> MSAPTPLAEASQIPTIPALSPLTAKQSKGNFFSSNPISSFVVDTYKQLHSHRQSLELVNPGTVENLNK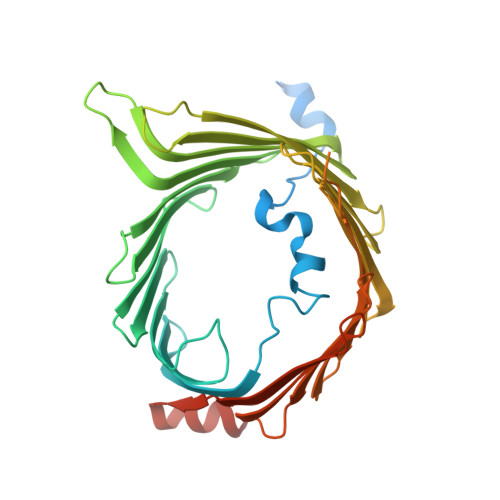EVSRDVFLSQYFFTGLRADLNKAFSMNPAFQTSHTFSIGSQALPKYAFSALFANDNLFAQGNIDNDLSVSGRLNYGWDKKNISKVNLQISDGQPTMCQLEQDYQASDFSVNVKTLNPSFSEKGEFTGVAVASFLQSVTPQLALGLETLYSRTDGSAPGDAGVSYLTRYVSKKQDWIFSGQLQANGALIASLWRKVAQNVEAGIETTLQAGMVPITDPLMGTPIGIQPTVEGSTTIGAKYEYRQSVYRGTLDSNGKVACFLERKVLPTLSVLFCGEIDHFKNDTKIGCGLQFETAGNQELLMLQQGLDADGNPLQALPQL>[2x]GPLGSSKVSEQLKCCSGILKEMFAKKHAAYAWPFYKPVDVEALGLHDYCDIIKHPMDMSTIKSKLEAREYRDAQEFGADVRLMFSNCYKYNPPDHEVVAMARKLQDVFEMRFAKM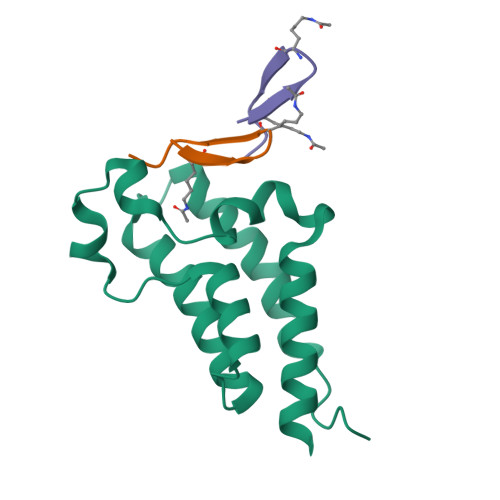PDEPEEP;>[3x]WKYWRKYVLKIC>[2x]MTEETISQAVPPVRDWPAVDLPGSDFDPVLTELMREGPVTRISLPNGEGWAWLVTRHDDVRLVTNDPRFGREAVMDRQVTRLAPHFIPARGAVGFLDPPDHTRLRRSVAAAFTARGVERVRERSRGMLDELVDAMLRAGPPADLTEAVLSPFPIAVICELMGVPATDRHSMHTWTQLILSSSHGAEVSERAKNEMNAYFSDLIGLRSDSA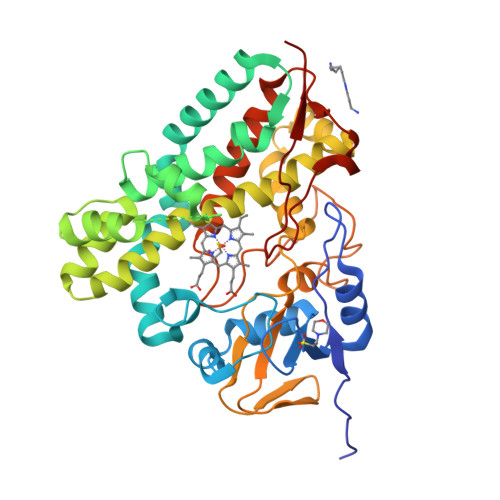GEDVTSLLGAAVGRDEITLSEAVGLAVLLQIGGEAVTNNSGQMFHLLLSRPELAERLRSEPEIRPRAIDELLRWIPHRNAVGLSRIALEDVEIKGVRIRAGDAVYVSYLAANRDPEVFPDPDRIDFERSPNPHVSFGFGPHYCPGGMLARLESELLVDAVLDRVPGLKLAVAPEDVPFKKGALIRGPEALPVTWHH> SPNVEACGYSDRVLQLTLGNSTITTQEAANSVVAYGRWPEFIRDDEANPVDQPTEPDVATCRFYTLDTVMWGKESKGWWWKLPDALRDMGLFGQNMYYHYLGRSGYTVHVQCNASKFHQGALGVFAIPEYCLAGDSDKQRYTSYANANPGERGGKFYSQFNKDNAVTSPKREFCPV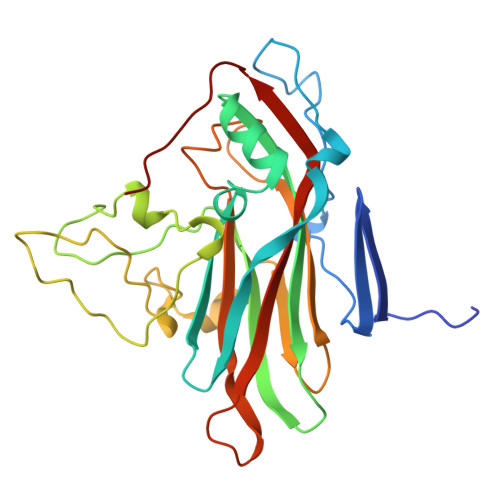DYLLGCGVLLGNAFVYPHQIINLRTNNSATIVLPYVNALAIDSMVKHNNWGIAILPLSPLDFAQDSSVEIPITVTIAPMCSEFNGLRNVTAPKFQ>MGRIKNKQFAVIGLGRFGGSICKELHRMGHEVLAVDINEEKVNAYASYATHAVIANATEENELLSLGIRNFEYVIVAIGANIQASTLTTLLLKELDIPNIWVKAQNYYHHKVLEKIGADRIIHPQKDMGVKIAQSLSDENVLNYIDLSDEYSIVELLATRKLDSKSIIDLNVRAKYGCTILAIKHHGDICLSPAPEDIIREQDCLVIMGHKKDIKRFENEGM[8x]

KtrAB is a cation channel with a nucleotide-dependent RCK domain. The structure of the KtrAB complex revealed a homodimeric membrane protein (KtrB) assembled with a cytosolic RCK octameric ring, formed by the KtrA protein. KtrA binds nucleotides, ATP or ADP. ATP binding induces the adoption of a square-conformation by the octameric ring and increased K+ flux activity through KtrAB; ADP binding results in a non-square conformation and decreased flux.

We introduced the single-point mutations R16A, R16K, A80P and E125Q in KtrA and tested their impact in the complementation assay. However, and contrary to our predictions, none of the R16 mutations had an impact on the growth phenotype, while E125Q resulted in an apparently inactive KtrAB. Crystal structures of the mutants that did not rescue the TK2420 growth phenotype (A80P and E125Q) reveal a different picture. The ATP-bound structures do not adopt a square conformation, displaying L1/L2 distances for A80P (at 3.9 Å resolution) of 52/23 Å and for E125Q (at 4.1 Å resolution and with two different half-rings in the asymmetric unit) of 34/30 Å and 42/27 Å. The ADP-bound structures are also non-square, showing ring conformations that are very similar to those observed with ATP: A80P (at 4.3 Å resolution) has L1/L2 distances of 52/22 Å and E125Q (at 4.0 Å resolution and with two rings) of 34/30 Å and 42/27 Å. In contrast, we found a large structural variability in the non-square structures, with four different conformational groups based on Cα N38 L1/L2 distances. This indicates that there is a single well defined square or active conformation for KtrA, while the ring in the non-active (or non-square) conformation is most likely more flexible, giving rise to different ring conformations in the crystals of isolated KtrA.>SMTIGRAKVYATLSKIFYHLFYDEAIPKDCREIIEKFGEIDFNLRSVLVRELRGSVLIKDMPQSLAEVYESVMKDFYER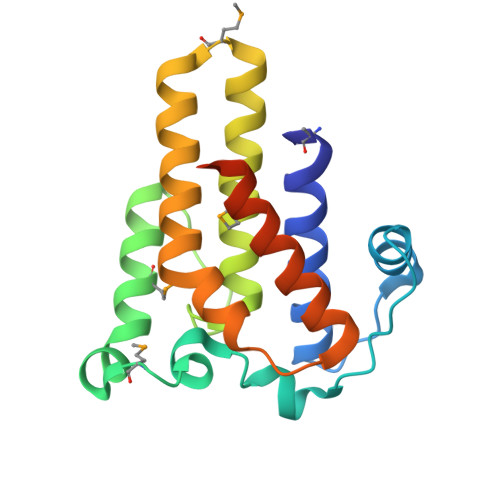YGFQASELHADHIAVELAFMSKLVEREISLAQQMKEEELYKIRAAQHRFIKAHLQPLVKNLPSAPLLNFVRDFVREDAKYLYSSLVGEKNEGADNN[3x]>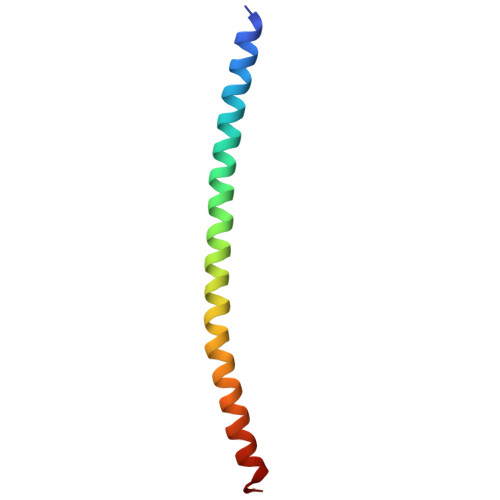 MFMKEKLLAELEGKLRVFENIVAVLNKEVEASHLALATSIHQSQLDRERILSLEQRVVELQQTLA> SMGKKSRVKTQKSGTGATATVSPKEILNLTSELLQKCSSPAPGPGKEWEEYVQIRTLVEKIRKKQKGLSVTFDGKREDYFPDLMKWASENGASVEGFEMVNFKEEGFGLRATRDIKAEELFLWVPRKLLMTVESAKNSVLGPLYSQDRILQAMGNIALAFHLLCERASPNSFWQPYIQTLPSEYDTPLYFEEDEVRYLQS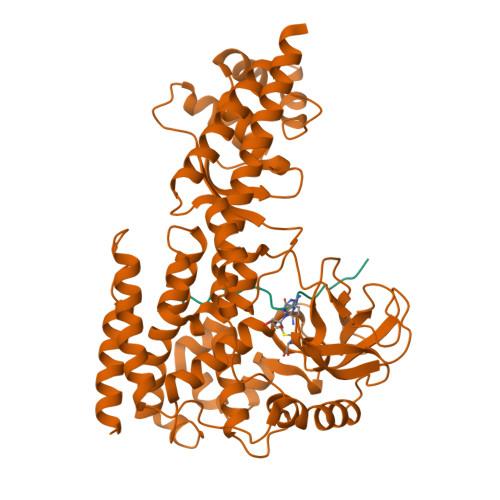TQAIHDVFSQYKNTARQYAYFYKVIQTHPHANKLPLKDSFTYEDYRWAVSSVMTRQNQIPTEDGSRVTLALIPLWDMCNHTNGLITTGYNLEDDRCECVALQDFRAGEQIYIFYGTRSNAEFVIHSGFFFDNNSHDRVKIKLGVSKSDRLYAMKAEVLARAGIPTSSVFALHFTEPPISAQLLAFLRVFCMTEEELKEHLLGDSAIDRIFTLGNSEFPVSWDNEVKLWTFLEDRASLLLKTYKTTIEEDKSVLKNHDLSVRAKMAIKLRLGEKEILEKAVKSAAVNREYYRQQMEEKAP;> TLKYPIEAGIVTNWDD1-((1R)-1-(HYDROXYMETHYL)-3-(1-NAPHTHYL)PROPYL)-1H-IMIDAZOLE-4-CARBOXAMIDE | C18 H19 N3 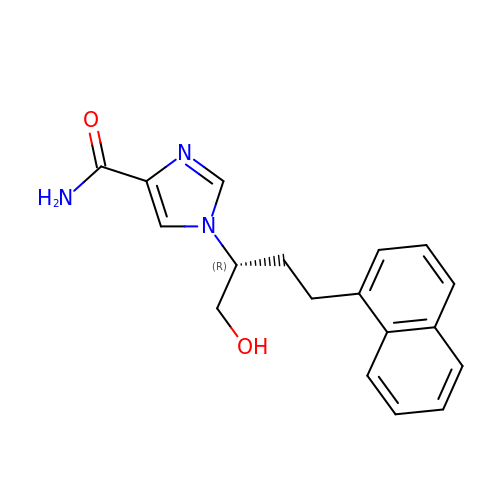O2 | URGFTPMACWKJKU-OAHLLOKOSA-N>[2x]PISADFSEVENAPSFLSLAENTDEVLKPYTGLEIQTIITNIVGDANPNQSRIFDQDRLRGNQYSAGGLVTQNAVSAIPFTNLIPRTIRVGNILVNSANRLQITETNVSEYYSNPIIATKLSEMISDQVKNNQFSTWRRDNTSLQGFNAFDIATINTAILPNGLSLESMLLKLSLLHSIKAMNVDAASINRSQYQVIDHNTVPTIGAPAVVGVNNSPVFGEDCGGNNPVYPFGGGTGAIAFHVTLQTVPDERKSYAIFVPPAILQATSDANEALALFALSMSEWPHALYTVTKQTTDLAGANAGQQVFIPTQSTIHIGGRRVLDLIIPRREIAPNPTTLVAANAMCMVRPQAGPDATAGAIPLAAGQLFNMNFIGAPAFEEWPMTSYLYSWAGRFDITTIRQYMGRLATMVGVKDAYWAAHELNVALSQVAPKMTTAAGGWAAQAANSAQQSDVCYSSLLTVTRSAANFPLANQPAADMRVYDTDPATWNKVALGLATAANLVPEQSMDVPFVVGDARASFWERLQAIPMCIAWTMYYHSRGITTLAWDNAYTDNTNKWLQKMVRNTFSTTQSVGTIIPARYGKIVCNLYKNMFHRAPAYVATSVGGKELHITHFERWLPGGTYANVYSGAGAVVNCFSPVLIPDIWCQYFTAKLPLFAGAFPPAQGQNSTKGFNSKQGLMIHRNQNNNLVAPYLEKFADNSSYFPVGQGPEINDMATWNGRLWMTTGNVQYLDYSGAAIVEAVPPAGELPVGKQIPLLAGENAPIELTNAATTCVPRYSNDGRRIFTYLTTAQSVIPVQACNRAANLARSCWLLSNVYAEPALQALGDEVEDAFDTLTNSSFLDVAKSVAESAGEVPATKALTDLQAVDVSSLPSTSDPSNVLSQPAPLMSPPTSSS

Recently, several unassigned viruses isolated from mosquitoes, including the Omono River virus (OmRV), were identified as totivirus-like viruses, with features similar to those of the Totiviridae family. Here, we identified a new strain of OmRV and determined high-resolution structures for this virus using single-particle cryo-electron microscopy. Generally, members of Totiviridae and totivirus-like viruses have a non-segmented double-stranded RNA (dsRNA) genome containing two large overlapping open reading frames (ORFs), namely, ORF1 and ORF2, which encode the major capsid protein (MCP) and RNA-dependent RNA polymerase (RdRP), respectively. Similar to that of other members of Totiviridae, OmRV-LZ has a major capsid with icosahedral symmetry and a T = 1 lattice comprising 60 dimers composed of MCP-A and MCP-B. The central cross-sectional view of the map with the genome shows at least five visible layers of viral genome RNA packaged inside the capsid.

The final two three-dimensional (3-D) maps were resolved at 2.79 Å (full particles with genome) and 3.40 Å (empty particles without genome), respectively, based on the Fourier shell correlation (FSC) 0.143 criterion. The current resolution of the map for the full particle allows us to build ab initio atomic models of the MCPs. In each asymmetric unit, MCP-A and MCP-B share a similar tertiary structure, and the overall structures of these two subunits are well aligned with each other, showing a root mean square deviation (RMSD) of 0.66 Å for 728 Cα atom pairs. Each MCP-A is located close to the five-fold vertex, while MCP-B fills the vicinity of the three-fold axis. The ab initio models revealed that the first residue of the N-terminus of both MCP-A and MCP-B was clearly located at Pro789, which provides strong evidence for cleavage at CM-1 between residues Asn788 and Pro789 in OmRV. The C-terminal residues 1641–1685 of MCP-A are disordered. The MCP-B C-terminal residues 1618–1682 form a Ω-like arm structure composed of four loops and three α-helices. It extends along the interface between MCP A-B-A and interacts extensively with two neighbouring MCP-As. All these MCP A-B-A interactions strongly fasten the capsid decamer around the five-fold axis. However, in OmRV-LZ, the C-terminus of MCP-B, instead of N-terminus, play roles in stabilizing the capsid.> MKKEVRKVRIALASPEKIRSWSYGEVEKPETINYRTLKPERDGLFDERIFGPIKDYECACGKYKRQRFEGKVCERCGVEVTKSIVKRYRMGHIELATPAAHIWFVKDVPSKIGTLLDLSATELEQVLYFSKYIVLDPKGAILNGVPVEKRQLLTDEEYRELRYGKQETYPLPPGVDALVKDGEEVVKGQELAPGVVSRLDGVALYRFPRRVRVEYVKKERAGLRLPLAAWVEKEAYKPGEILAELPEPYLFRAEEEGVVELKELEEGAFLVLRREDEPVATYFLPVGMTPLVVHGEIVEKGQPLAEAKGLLRMPRQVRAAQVEAEEEGETVYLTLFLEWTEPKDYRVQPHMNVVVPEGARVEAGDKIVAAIDPEEEVIAEAEGVVHLHEPASILVVKARVYPFEDD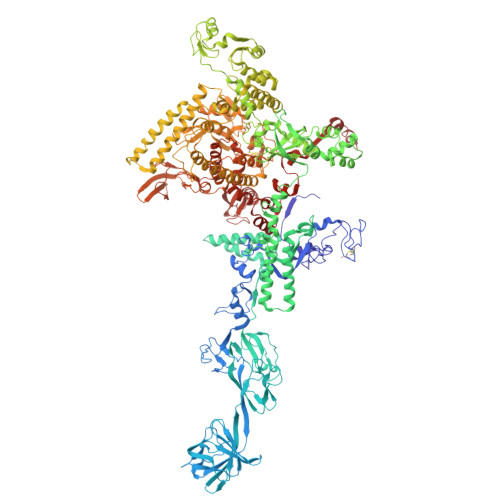VEVSTGDRVAPGDVLADGGKVKSDVYGRVEVDLVRNVVRVVESYDIDARMGAEAIQQLLKELDLEALEKELLEEMKHPSRARRAKARKRLEVVRAFLDSGNRPEWMILEAVPVLPPDLRPMVQVDGGRFATSDLNDLYRRLINRNNRLKKLLAQGAPEIIIRNEKRMLQEAVDALLDNGRRGAPVTNPGSDRPLRSLTDILSGKQGRFRQNLLGKRVDYSGRSVIVVGPQLKLHQCGLPKRMALELFKPFLLKKMEEKGIAPNVKAARRMLERQRDIKDEVWDALEEVIHGKVVLLNRAPTLHRLGIQAFQPVLVEGQSIQLHPLVCEAFNADFDGDQMAVHVPLSSFAQAEARIQMLSAHNLLSPASGEPLAKPSRDIILGLYYITQVRKEKKGAGLEFATPEEALAAHERGEVALNAPIKVAGRETSVGRLKYVFANPDEALLAVAHGIVDLQDVVTVRYMGKRLETSPGRILFARIVAEAVEDEKVAWELIQLDVPQEKNSLKDLVYQAFLRLGMEKTARLLDALKYYGFTFSTTSGITIGIDDAVIPEEKKQYLEEADRKLLQIEQAYEMGFLTDRERYDQILQLWTETTEKVTQAVFKNFEENYPFNPLYVMAQSGARGNPQQIRQLCGLRGLMQKPSGETFEVPVRSSFREGLTVLEYFISSHGARKGGADTALRTADSGYLTRKLVDVTHEIVVREADCGTTNYISVPLFQPDEVTRSLRLRKRADIEAGLYGRVLAREVEVLGVRLEEGRYLSMDDVHLLIKAAEAGEIQEVPVRSPLTCQTRYGVCQKCYGYDLSMARPVSIGEAVGIVAAQSIGEPGTQLTMRTFHTGGVAGAADITQGLPRVIELFEARRPKAKAVISEIDGVVRIEETEEKLSVFVESEGFSKEYKLPKEARLLVKDGDYVEAGQPLTRGAIDPHQLLEAKGPEAVERYLVEEIQKVYRAQGVKLHDKHIEIVVRQMMKYVEVTDPGDSRLLEGQVLEKWDVEALNERLIAEGKTPVAWKPLLMGVTKSALSTKSWLSAASFQNTTHVLTEAAIAGKKDELIGLKENVILGRLIPAGTGSDFVRFTQVVDQKTLKAIEEARKEAVEA> EDPVTGPEEVSGQEQGSLTVQCRYTSGWKDYKKYWCQGVPQRSCK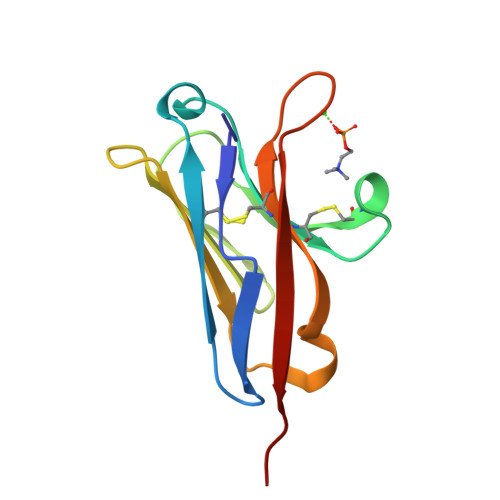TLVETDASEQLVKKNRVSIRDNQRDFIFTVTMEDLRMSDAGIYWCGITKGGLDPMFKVTVNIGPVP>MARFNAAFTRIKIMFSRIRGLISCQSNTQTIAPTLSPPSSGHVSFAGIDYPLLPLNHQTPLVFQWFERNPDRFGQNEIPIINTQKNPYLNNIINAAIIEKERIIGIFVDGDFSKGQRKALGKLEQNYRNIKVIYNSDLNYSMYDKKLTTIYLENITKLEAQSASERDEVLLNGVKKSLEDVLKNNPEETLISSHNKDKGHLWFDFYRNLFLLKGSDAFLEAGKPGCHHLQPGGGCIYLDADMLLTDKLGTLYLPDGIAIHVSRKDNHVSLENGIIAVNRSEHPALIKGLEIMHSKPYGDPYNDWLSKGLRHYFDGSHIQDYD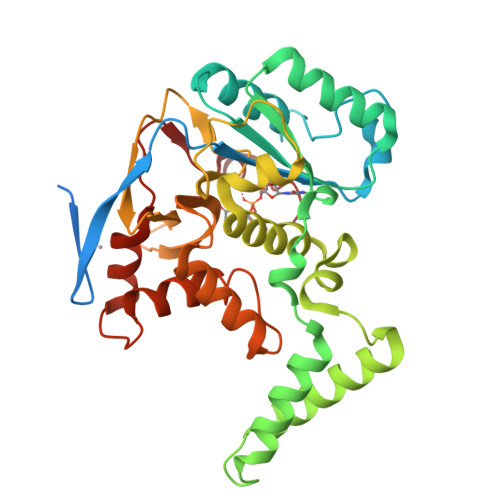AFCDFIEFKHENIIMNTSSLTASSWR[4x]> ENLYFQGMRFVVALTGASGQILGIRLIEKLTELGAEVYAVASRAAKITLKAETDYDEGYVREIATKYYDEDEIAAP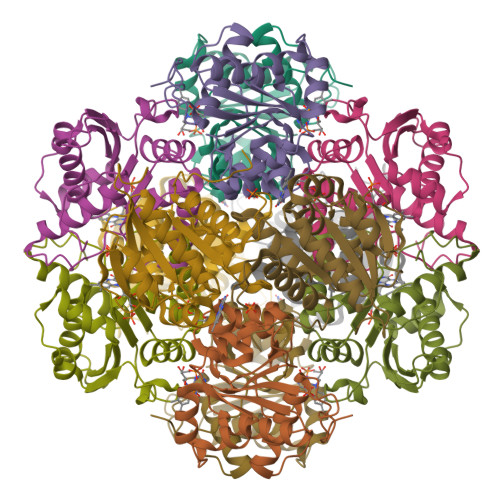FASGSFRHDGMAVVPCSIKTASSIAYGIADNLIARAADVTLKEKRRLVLAIREAPLHSGHLKTLARLAEMGAVIFPPVLSFYTRPKSVDDLIEHTVSRIAEQLGVEVDYRRWG> LGKFSQTCYNSAIQGSVLTSTCERTNGGYNTSSIDLNSVIAAVDGS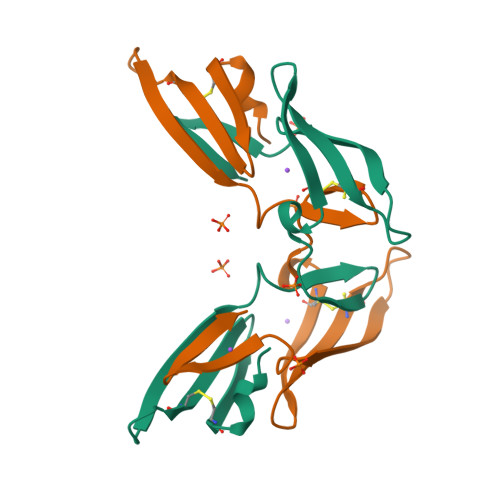LKWPSNFIEACRNTQLAGSSELAAECKTAAGQFVSTKINLDDHIANIDGTLKYE>MKVTYSGSDSKTYDGNPANFEPTTVQWSGLKGLNTSTLTSADFTWNTADKKAPTDAGKYTLSLNTTGE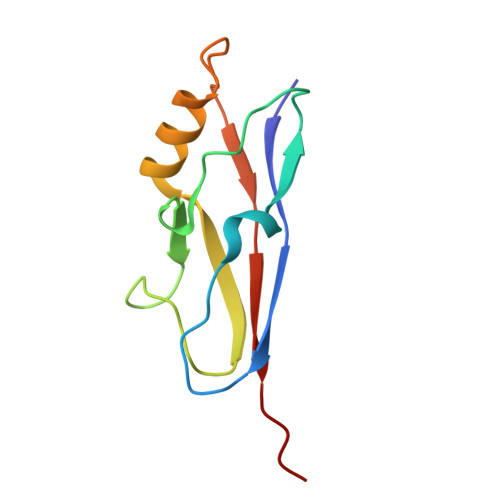AALRKANPNYDLKTISGSYTYTINPLGID[3x]>MRAVRLVEIGKP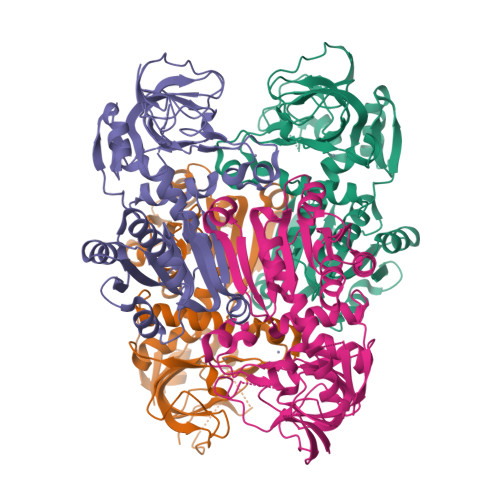LSLQEIGVPKPKGPQVLIKVEAAGVCHSDVHMRQGRFGNLRIVEDLGVKLPVTLGHEIAGKIEEVGDEVVGYSKGDLVAVNPLQGEGNCYYCRIGEEHLCDSPRWLGINFDGAYAEYVIVPHYKYMYKLRRLNAVEAAPLTCSGITTYRAVRKASLDPTKTLLVVGAGGGLGTMAVQIAKAVSGATIIGVDVREEAVEAAKRAGADYVINASMQDPLAEIRRITESKGVDAVIDLNYSEKTLSVYPKALAKQGKYVMVGLFGADLHYHAPLITLSEIQFVGSLVGNQSDFLGIMRLAEAGKVKPMITKTMKLEEANEAIDNLENFKAIGRQVLIP[6x]>VGLRRRARLSRLVSFSASHRLHSPSLSAEENLKVFGKCN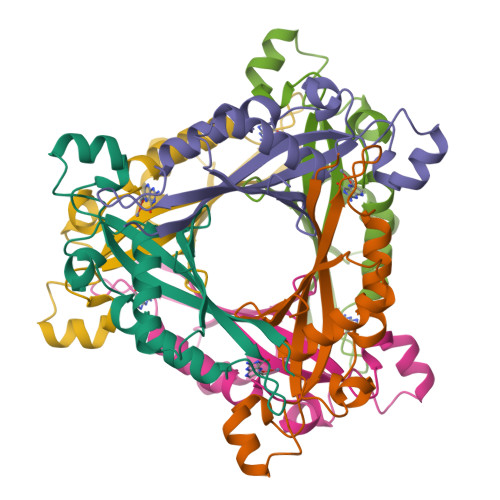NPNGHGHNYKVVVTIHGEIDPVTGMVMNLTDLKEYMEEAIMKPLDHKNLDLDVPYFADVVSTTENVAVYIWENLQRLLPVGALYKVKVYETDNNIVVYKGE[2x]(3S)-3-[2-(1,3-benzodioxol-5-yl)-2-oxidanylidene-ethyl]-4-bromanyl-5-methyl-3-oxidanyl-1H-indol-2-one | C18 H14 Br N O5 | 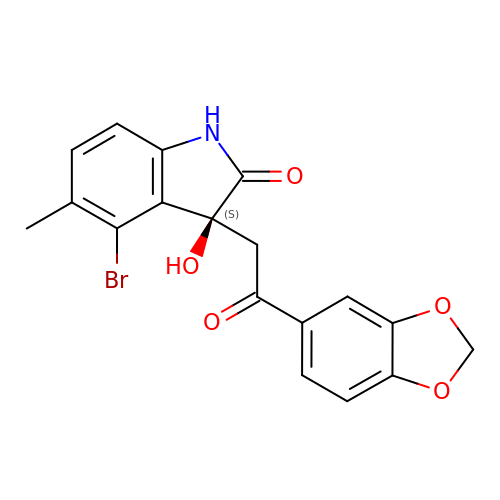SJXSNMXBXJIRLV-SFHVURJKSA-N The disassembly of ESCRT-III is mainly mediated by the Vps4 protein that is a member of the type I AAA+ ATPase (ATPase associated with various cellular activities) family and oligomerizes into a functional hexamer with elevated ATPase activity upon binding to ATP6. Powered by ATP hydrolysis, the Vps4 oligomer, promoted by the cofactor protein Vta1 (Vps twenty associated 1), disassembles ESCRT-III polymers into individual ESCRT-III subunits available for recycling. Vps4 protein contains an MIT (microtubule interacting and trafficking) domain at the N terminus, a single ATPase cassette comprising a large ATPase domain and a small ATPase domain with a β-domain inserted within it, and a C-terminal helix8111213. In this study, using Vps4 from yeast, we solved the structures of the ATP-bound Vps4E233Q hexamer at 3.9 Å resolution and its complex with Vta1 at 4.2 Å resolution, both determined by single-particle electron cryo-microscopy (cryo-EM) without any symmetry imposed.

We purified the full-length yeast Vps4 containing an E233Q mutation, which allows ATP binding but blocks ATP hydrolysis, and assembled Vps4E233Q oligomer in the presence of 1 mM ATP in vitro. We used single-particle cryo-EM method to obtain the three-dimensional (3D) reconstruction of the 300 kDa oligomer without imposing any symmetry at a resolution of 3.9 Å. The structure appeared as a hexameric ring, consistent with the MALS result. Although we used the full-length Vps4E233Q for the oligomer assembly and the Vps4E233Q protein in the hexamer was intact as evidenced by the SDS–polyacrylamide gel electrophoresis (SDS–PAGE) gel showing a molecular weight of ∼50 kD, the six MIT domains exhibit no EM density, likely reflecting their dynamic locations due to the long linker of ∼40 residues between the MIT domain and the followed ATPase cassette (upper). The subunit A shifts slightly away from the ring centre, and the interaction interfaces between it and its two adjacent subunits are only about half of those between the other subunits. Moreover, the ring is not planner, in which subunits arrange in an upward spiral from subunit A to subunit F as manifested by the relative positions of the α3-helix and C-terminal helix in each subunit, resembling a split right-handed spiral ring. Agreeing with this, densities for nucleotides are clearly visible in the nucleotide-binding pockets of subunit B through F, whereas there is no clear density in the nucleotide-binding pocket of subunit A, suggesting that subunit A is likely free of the nucleotide. The inter-subunit interactions occur both between the large ATPase domains and between the large ATPase and the small ATPase domains including the β-domain.

>MSTGDFLTKGIELVQKAIDLDTATQYEEAYTAYYNGLDYLMLALKYEKNPKSKDLIRAKFTEYLNRAEQLKKHLESEEANAAKKSPSAGSGSNGGNKKISQEEGEDNGGEDNKKLRGALSSAILSEKPNVKWEDVAGLEGAKEALKEAVILPVKFPHLFKGNRKPTSGILLYGPPGTGKSYLAKAVATEANSTFFSVSSSDLVSKWMGESEKLVKQLFAMARENKPSIIFIDQVDALTGTRGEGESEASRRIKTELLVQMNGVGNDSQGVLVLGATNIPWQLDSAIRRRFERRIYIPLPDLAARTTMFEINVGDTPCVLTKEDYRTLGAMTEGYSGSDIAVVVKDALMQPIRKIQSATHFKDVSTEDDETRKLTPCSPGDDGAIEMSWTDIEADELKEPDLTIKDFLKAIKSTRPTVNEDDLLKQEQFTRDFGQEGN[6x]> MCFSPKIKTPKMDTNQIRAV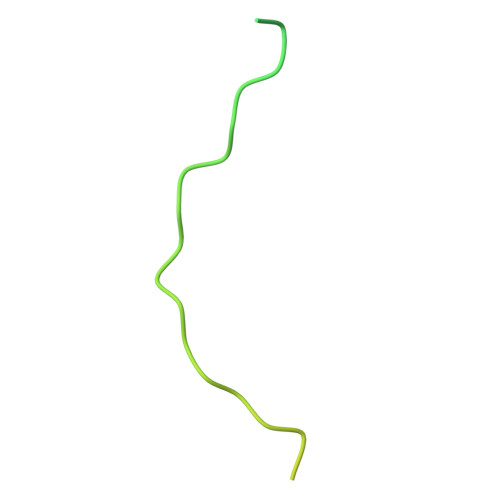EPAPLTQEVSSVEFGGSSDETDTEGTEVSGRKGLKVERDDSVAKSKASGNGSARMKSSIRKSAFGGKK>[4x]HHHHHHMRVILDGCSLTPDVLYALGYEKGATIEISDEAVARITAARAVIDKIVNDRQTVYGINTGFGKFESTIIPPHQLEELQLNLIRSHSACVGEPLTPERARMMLALRVNVLCKGHSGIRLETVQKYLKAFNAGVVPYIPEQGTVGASGDLGPLSHLALGMLGEGLLATLNNKKFRDAGSVLRELGVEPITLAAKEGLALINGTQFISALGAEAVVRARKIARLADVALAMSHEALRATNSTLNPDIHRVRPHKGQQLVAQRLRALLHSEEYPSMINESHVNCGRVQDAYSIRCAPQVHGISNEVIEWVYGILTTELNCATDNPLVFPDGVKKVVSGGNFHGEYPAKALDMLAIGVHELGNISERRIERLNNPTLSRLPAFLVKNGGLNSGFMIAHCTAAALVSENKVYCHPASADSISTSAAQEDHVSMGGFSARKAIKVVENVERIIAIELLGACQGIDLLRPLRTTEPMEKVWSLVRSVSPPWEEDRVINTDIDNVT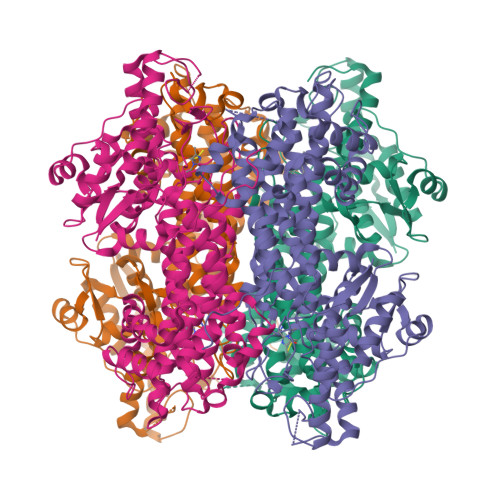KLLRSGAVWKTVKPYVPEEARFLGVLTVKKPFELKSKM>[2x]SKDRISWLGQPMKIEENRTYYQKVSIDEEMLEVGDCVSVIPDDSSK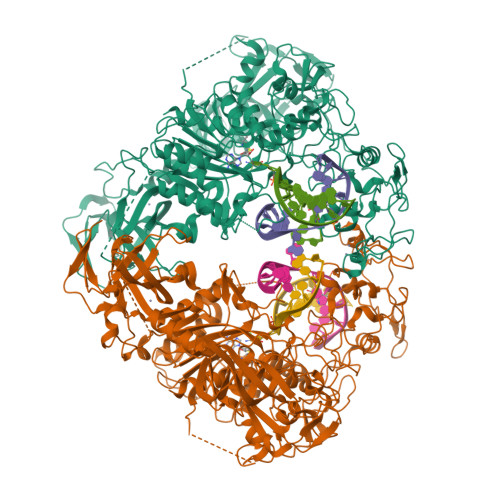PLYLARVTALWEDKNGQMMFHAHWFCAGTDTVLGATSDPLELFLVGECENMQLSYIHSKVKVIYKAPSENWAMEGGTDPETTLPGAEDGKTYFFQLWYNQEYARFESPPKTQPTEDNKHKFCLSCIRLAELRQKEMPKVLEQIEEVDGRVYCSSITKNGVVYRLGDSVYLPPEAFTFNIKVASPVKRPKKDPVNETLYPEHYRKYSDYIKGSNLDAPEPYRIGRIKEIHCGKKKGKVNEADIKLRLYKFYRPENTHRSYNGSYHTDINMLYWSDEEAVVNFSDVQGRCTVEYGEDLLESIQDYSQGGPDRFYFLEAYNSKTKNFEDPPNHARSPGNKGKGKGKGKGKGKHQVSEPKEPEAAIKLPKLRTLDVFSGCGGLSEGFHQAGISETLWAIEMWDPAAQAFRLNNPGTTVFTEDCNVLLKLVMAGEVTNSLGQRLPQKGDVEMLCGGPPCQGFSGMNRFNSRTYSKFKNSLVVSFLSYCDYYRPRFFLLENVRNFVSYRRSMVLKLTLRCLVRMGYQCTFGVLQAGQYGVAQTRRRAIILAAAPGEKLPLFPEPLHVFAPRACQLSVVVDDKKFVSNITRLSSGPFRTITVRDTMSDLPEIQNGASNSEIPYNGEPLSWFQRQLRGSHYQPILRDHICKDMSPLVAARMRHIPLFPGSDWRDLPNIQVRLGDGVIAHKLQYTFHDVKNGYSSTGALRGVCSCAEGKACDPESRQFSTLIPWCLPHTGNRHNHWAGLYGRLEWDGFFSTTVTNPEPMGKQGRVLHPEQHRVVSVRECARSQGFPDSYRFFGNILDRHRQVGNAVPPPLAKAIGLEIKLCLLSSA> MNMFFRLTALAGLLAIAGQTFAVEDITRADQIPVLKEETQHATVSERVTSRFTRSHYRQFDLDQAFSAKIFDRYLNLLDYSHNVLLASDVEQFAKKKTELGDELRSGKLDVFYDLYNLAQKRRFERYQYALSVLEKPMDFTGNDTYNLDRSKAPWPKNEAELNALWDSKVKFDELSLKLTGKTDKEIRETLTRRYKFAIRRLAQTNSEDVFSLAMTAFAREIDPHTNYLSPRNTEQFNTEMSLSLEGIGAVLQMDDDYTVINSMVAGGPAAKSKAISVGDKIVGVGQTGKPMVDVIG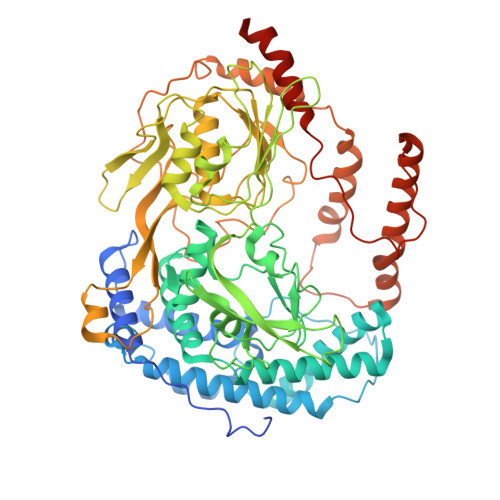WRLDDVVALIKGPKGSKVRLEILPAGKGTKTRTVTLTRERIRLEDRAVKMSVKTVGKEKVGVLDIPGFYVGLTDDVKVQLQKLEKQNVSSVIIDLRSNGGGALTEAVSLSGLFIPAGPIVQVRDNNGKVREDSDTDGQVFYKGPLVVLVDRFSAAASEIFAAAMQDYGRALVVGEPTFGAGTVQQYRSLNRIYDQMLRPEWPALGSVQYTIQKFYRVNGGSTQRKGVTPDIIMPTGNEETETGEKFEDNALPWDSIDAATYVKSGDLTAFEPELLKEHNARIAKDPEFQNIMKDIARFNAMKDKRNIVSLNYAVREKENNEDDATRLARLNERFKREGKPELKKLDDLPKDYQEPDPYLDETVNIALDLAKLEKARPAEQPAPVKHHHHHH methyl 1H-indole-3-carboxylate | C10 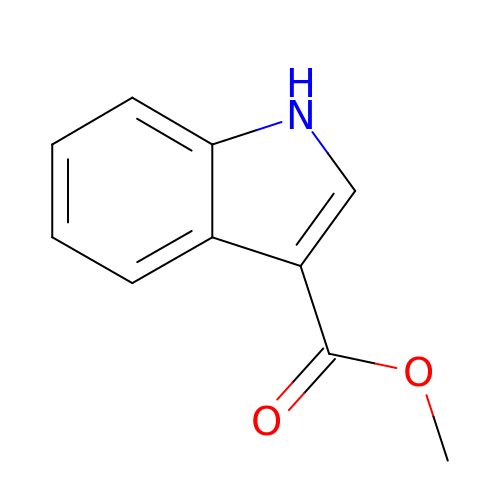H9 N O2 | QXAUTQFAWKKNLM-UHFFFAOYSA-N> VMTMRGLLVGKMQPFHRGHLQVIKSILEEVDELIICIGSAQLSHSIRDPFTAGERVMMLT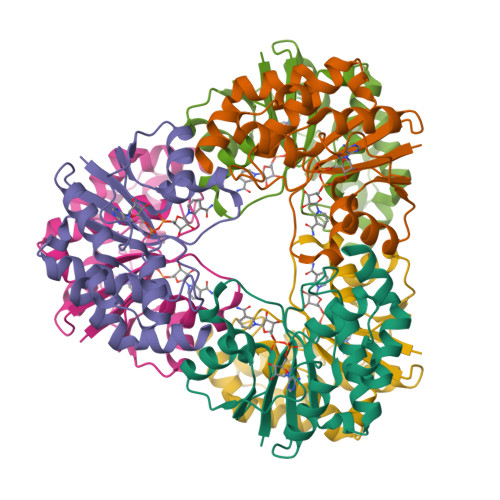KALSENGIPASRYYIIPVQDIECNALWVGHIKMLTPPFDRVYSGNPLVQRLFSEDGYEVTAPPLFYRDRYSGTEVRRRMLDDGDWRSLLPESVVEVIDEINGVERIKHLAKKEVSELGGIS The ketol-acid reductoisomerase (KARI, EC 1.1.1.86) catalyses the reversible conversion of acetohydroxy acids into the corresponding hydroxyl valerates, a crucial step in the biosynthesis pathway of valine, leucine and isoleucine. KARIs are structurally composed of an N-terminal Rossmann domain and a C-terminal “knot” domain. They can be distinguished in two classes: the short class I gathering dimeric and dodecameric enzymes, and the monomeric or tetrameric longer class II KARIs. Here we describe the structure of the purified native dodecameric enzyme from M. thermolithotrophicus (referred here as MtKARI), which is the first structurally characterised KARI from a methanogen.

X-ray diffraction measurements were initially performed on crystals obtained from MtKARI purified and crystallised without any additional ions or substrates. The refinement and electron density quality was hampered by merohedral twinning, with a very high fraction (0.32); however, the model was complete and was refined to a 2.1-Å resolution. The overall conformation of the enzyme fits the well-characterised close state. In the obtained close state of MtKARI, NADP and Mg2+ are bound in the structure, even though we did not add any ligands in the crystallisation and soaking solutions. They therefore were natively co-purified from the cells of M. thermolithotrophicus. The structure of MtKARI in the close state harbours NADPH or NADP+ (later mentioned as NADP for convenience) bound to the Rossmann domain, as well as two metals coordinated at the Mg2+ binding site in structurally characterised homologs. While the NADP has a proper fit in the electron density, the suspected Mg2+ ions have a lower occupancy, especially for the second site, which might come from the twinning or a rather loose hexacoordination for the second site (site B). The first Mg2+ (site A) is hexacoordinated by Glu195, Asp191 and four waters, while the second ion (site B) is coordinated by Asp191, Glu231 and four water molecules with a far distant interaction with Glu227. The Arg48 and Ser53 selectively accommodate and stabilise the 2′-phosphate of NADP in the close state, similar to what is observed in SlaeKARI; however, the second stabilising serine (Ser61 in SlaeKARI) does not exist in MtKARI. A hydrophobic pocket contains the adenine moiety, several hydrogen bonds bind the pyrophosphate to the protein backbone and the ribose-nicotinamide part is bound by Asp83, Gly134 and a water network.

> MMKVFYDSDTTFDAVKDKTIAVIGYGSQGRAQSLNMKDSGLKVVVGLRPNGASWNKAKEDGHEVLSIEEAAEKADIIHILIPDEIQGDVYNKQIKPYLKEGKTLSFSHGYNIHYGYIVPPEGVNVVMVAPKSPGAMVRRTYEEGFGVPGLVCVEKDATGDALDIALGMAKGVGLTRAGVIQTTFREETETDLFGEQAVLCGGVTELIKAGFETLVEAGYSPEMAYFETCHELKLIIDLIYQKGFAGMWNDVSNTAEYGGLTRRSRVINEQSRQEMRKILKEIQDGRFTKEWALENISGKAHLNSMRRIESELLIEEVGAKLRKMCGLQKD One especially common junction element is the kink-turn (k-turn). k-turns are elements in double-stranded RNA that introduce a tight kink into the helical axis, with an included angle close to 50°. A standard k-turn comprises a three-nucleotide bulge followed by successive G•A and A•G trans G(sugar edge)•A(Hoogsteen edge) basepairs. k-turns are commonly-occurring motifs that introduce sharp kinks into duplex RNA, thereby facilitating tertiary contacts. Both the folding and conformation of k-turns are determined by their local sequence. k-turns fall into two conformational classes, called N3 and N1, that differ in the pattern of hydrogen bonding in the core. We show here that this is determined by the basepair adjacent to the critical G•A pairs.

We therefore decided to extend the study with a systematic structural analysis of HmKt-7 as a function of the 3b,3n sequence. This was performed in the constant environment of the SAM-I riboswitch, modified by replacing its natural k-turn by HmKt-7 with different 3b,3n sequences. In this way we could observe the effect of changing the 3b,3n sequence alone in an otherwise completely unchanged RNA molecule. Additionally, we hoped we might expand the range of 3b,3n sequences beyond the eight found in the natural k-turns to date. Six are completely new, i.e. 3b,3n = C•A, C–G, C•U, G•G, U–A and U•C, five of which adopt the N1 conformation. Altogether seven of the new structures are in the N1 conformation, and clearly simply changing the 3b,3n sequence alone is sufficient to induce the structure of Kt-7 to change within the riboswitch environment. The N3 group contain a preponderance of 3b,3n = A•G and U•U pairs, and the N1 group comprise mainly 3b,3n = U•G, C•A and C•C pairs. Evidently the 3b,3n sequence is the major determinant of the k-turn conformation.

> GGCUUAUCAAGAGAGGGAGAGCGACUGGCGCGAAGACCCCCGGCAACCAGAAAUGGUGCCAAUUCCUGCAGCGGAAACGUUGAAAGAUGAGCCA>MNTEIISPHHYVYPNTTTLKNKYGIKNLNAFLEKCSHDTAKAMINLREESLPEYFDTAYLCHIHQQLFKNTFEWAGYL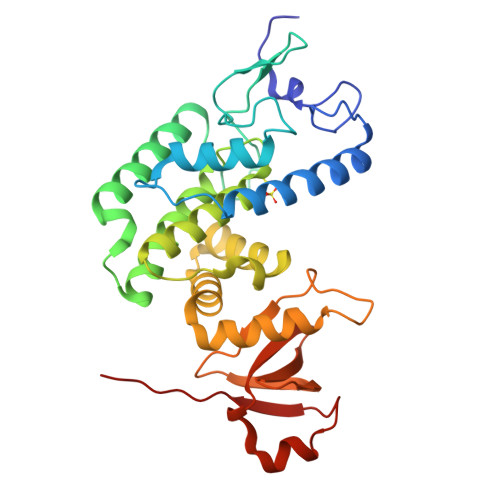RHIPFTFADGTTAAMPEMKRTGWKNAFAIGDEIQEGLQRLDQTLAEKNNLQGLTREEFNSEAIELFNSLNQLHPFREGNGRTQRLFFENLAKAAGHQLNFSLITKERMMVASVAVAENGDLEPMQHLFEDISNPEKIRLLKEFMHTMKNTGRNVNDRPVMVAKEGETYTGTYRGAGLEGFALNVKGAYIIGNIDHLPPEQLKILKPGDKITFTAPKAHHH[8x]>MATLEITDIALVQPSHQPLSNDQTLSLSHLDNDNNLHVSFRYLRVYSSSSSTVAGESPSAVVSASLATALVHYYPLAGSLRRSASDNRFELLCSAGQSVPLVNATVNCTLESVGYLDGPDPGFVERLVPDPTREEGMVNPCILQVTMFQCGGWVLGASIHHAICDGLGASLFFNAMAELARGATKISIEPVWDRERLLGPREKPWVGAPVRDFLSLDKDFDPYGQAIGDVKRDCFFVTDDSLDQLKAQLLEKSGLNFTTFEALGAYIWRAKVRAAKTEEKENVKFVYSINIRRLMNPPLPKGYWGNGCVPMYAQIKAGELIEQPIWKTAELIKQSKSNTSDEYVRSFIDFQ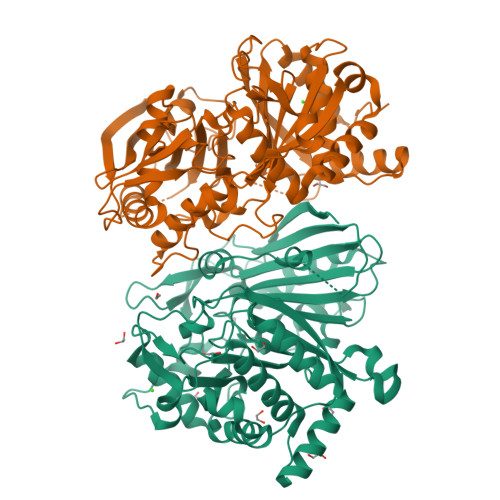ELHHKDGINAGTGVTGFTDWRYLGHSTIDFGWGGPVTVLPLSNKLLGSMEPCFFLPYSTDAAAGSKKDSGFKVLVNLRESAMPEFKEAMDKFHKGEFALS[2x]Bacterial-induced MNGC formation requires bacterial motility and the Type VI Secretion System cluster 1 (T6SS1, also known as T6SS5), one of the six T6SSs B. pseudomallei possesses. Hcp and VgrG (valine-glycine repeat protein G) are secreted substrates of T6SS that share homology with the bacteriophage tail and tail spike protein respectively, but they are also required for T6SS function. Hcp is required for both the assembly of a functional T6SS and the export of T6SS substrates by chaperoning the substrates, which includes itself. In this study, we have identified an extended loop region of Hcp1 (Loop L2, 3) that shows a significant movement away from the main Hcp β-barrel domain as compared to other known Hcp structures.

To understand the structure and function relationship of B. pseudomallei Hcp1, the crystal structure of recombinant Hcp1 was determined using the single wavelength anomalous diffraction method (SAD) with two molecules in the asymmetric unit. The model was refined to a final R-value of 0.248 (Rfree = 0.285) up to 2.7 Å resolution and has good stereo-chemical parameters. Each molecule of Hcp1 consists of a β-barrel domain, with several loops predominantly on one end of the β-barrel and an α-helix (Ser69 – Lys78) located on one side of the β-barrel. Notably, residues Asp40 to Arg56 form an extended loop (Loop L2, 3) that protrudes away from the β-barrel and is well defined in the electron density map. In particular, the major extended loop (Loop L2, 3) between Asp40 and Arg56 of Hcp1BP is significantly shifted by 18–20 Å relative to its homologs. In the crystals, the asymmetric unit consists of two Hcp1 molecules and the hexameric rings could be generated by a 6-fold symmetry with 12 molecules forming a two ring assembly. This stacking of hexameric rings could form the tube-like assembly with an outer diameter of 80 Å and an inner diameter of 40 Å. The symmetry related molecules of the hexameric ring show that the extended loop region of Hcp1 could potentially act as a key contact point between two hexameric rings. Most of them are hydrogen bond contacts involving the residues Gln46 to Thr50 from both interacting monomers of the stacked hexameric rings. AUC analysis showed that at 2 mg/mL, wildtype Hcp1 demonstrated two peaks corresponding to hexamers and dodecamers (black histogram) whereas Hcp1Q46AE47A exhibited a single peak that corresponded to hexamers (red histogram).

>[2x]MLAGIYLKVKGKTQGEIKGSVVQEGHDGKIHILAFKNDYDMPARLQEGLTPAAAARGTITLTKEMDRSSPQFLQALGKREMMEEFEITIHRPKTDTTGGDLTELLFTYKFEKVLITHMDQYSPTPHKDDSNGIKEGLLGYIEEIKFTYSGYSLEHAESGIAGAANWTNG> MHHHHHHENLYFQGTKDLNTLVSELPEIYQTIFGHPEWDGDAARDCNQRLDLITEQYDNLSRALGRPLNVLDLGCAQGFFSLSLASKGATIVGIDFQQENINVCRALAEENPDFAAEFRVGRIEEVIAALEEGEFDLAIGLSVFHHIVHLHGIDEVKRLLSRLADVTQAVILELAVKEEPFYWGVSQPDDPRELIEQCAFYRLIGEFDTHLSPVPRPMYLVSNHRVLINDFNQPFQHWQNQPYAGAGLAHKRSRRYFFGEDYVCKFFYYDMPHGILTAEESQRNKHELHNEIKFLTQPPAGFDAPAVLAHGENAQSGWLVMEKLPGRLLSDMLAAGEEIDREKILGSLLRSLAALEKKGFWHDDVRPWNVMVDARQHARLIDFGSIVTTPQDCSWPTNLVQSFFVFVNELFAENKSWNGFWRSAPVHPFNLPQPWSNWLYAVWQEPVERWNFALLLALFEKKAKLPSAEQQ

The chain length of the O9a O-PS is tightly regulated by the WbdD enzyme. WbdD first phosphorylates the terminal non-reducing mannose of the O-PS and then methylates the phosphate, stopping polymerization. The 82 kDa WbdD protein from E. coli O9a comprises 708 residues and contains three domains, an N-terminal methyltransferase (MTase) domain, a kinase domain and a C-terminal domain (residues 460–708) that includes predicted coiled-coil motifs. WbdD is an unusual enzyme since it combines both a phosphate-methyltransferase and a sugar kinase activity.

Removing this C-terminal helix (WbdD459) gave a monomeric protein in crystals (space group P212121) and in solution, confirming that the helical bundle drives trimer formation. The structures of WbdD459 and monomers of WbdD556 are very similar [r.m.s.d. = 1.5 Å (2538 superimposing atoms)], but there is a rigid-body rotation around the hinge connecting the N- and C-lobe within the kinase domain, accounting for the relatively large r.m.s.d. WbdD459, which lacks the C‐terminal bundle‐helix αV, showed a marked decrease in kinase activity but has lost the preference for 2α‐MB over d‐mannose. Thus, the C‐terminal bundle structure is clearly important both for biochemical activity and for polymer (substrate) recognition or co‐ordination. Of our structures, the ‘G-rich’ loop is most clearly defined in the Wbd459 structure, where it fulfils the same role as in Src; co-ordination of the AMPPNP (ATP mimic). However, in WbdD the loop protrudes further into the ATP binding cleft than the corresponding element in Src and it interacts with the catalytic loop through a π-stacking between W355 and Y230. WbdD binds ATP (or AMPPNP) via two Mg2+ ions (denoted Mg1, Mg2) that are co-ordinated by N356, D369 [part of the DFG motif which is almost universally conserved in kinases], E274 and all three phosphate groups of ATP (or AMPPNP), as well as by two water molecules. Mg1 bridges the α- and γ-phosphates, Mg2 the β- and γ-phosphates. We therefore attempted to co-crystallize WbdD556 and WbdD459 with d-mannose (KM > 100 mM) by soaking our crystals in saturated d-mannose solutions (∼ 1.6 M). Only WbdD459 crystals (with AMPPNP) withstood the treatment and gave additional electron density (not present before addition of d-mannose) that we interpret as two mannose units, Fig. 6A. The pocket is occupied by sulphate in the WbdD556 structure, these crystals were grown from ammonium sulphate solutions whereas the pocket is empty (with the loops disordered) in WbdD459 crystals which were grown from a non-sulphate-containing solution.3-[5-[(4~{a}~{R},8~{a}~{S})-4-oxidanylidene-3-propan-2-yl-4~{a},5,8,8~{a}-tetrahydrophthalazin-1-yl]-2-methoxy-phenyl]-~{N}-[2-(2-fluorophenyl)ethyl]prop-2-ynamide 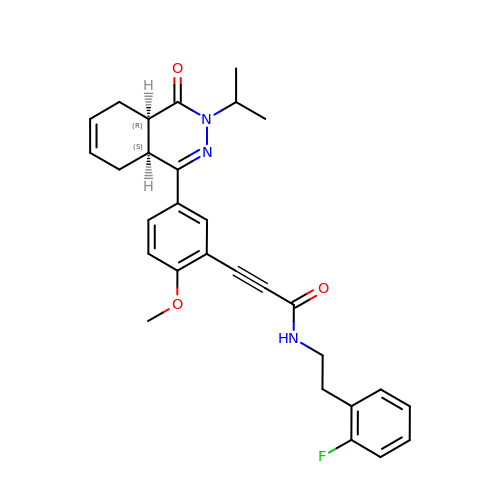| C29 H30 F N3 O3 | UAIXEGFVIVPDNH-BJKOFHAPSA-N> AGAIENARKEIKRISLEDHAESEYGAIYSVSGPVVIAENMIGCAMYELVKVGHDNLVGEVIRIDGDKATIQVYEETAGLTVGDPVLRTGKPLSVELGPGLMETIYDGIQRPLKAIKEESQSIYIPRGIDTPALDRTIKWQFTPGKFQVGDHISGGDIYGSVFENSLISSHKILLPPRSRGTITWIAPAGEYTLDEKILEVEFDGKKSDFTLYHTWPVRVPRPVTEKLSADYPLLTGQRVLDALFPCVQGGTTCIPGAFGCGKTVISQSLSKYSNSDAIIYVGCGERGNEMAEVLMEFPELYTEMSGTKEPIMKRTTLVANTSNMPVAAREASIYTGITLAEYFRDQGKNVSMIADSSSRWAEALREISGRLGEMPADQGFPAYLGAKLASFYERAGKAVALGSPDRTGSVSIVAAVSPAGGDFSDPVTTATLGITQVFWGLDKKLAQRKHFPSINTSVSYSKYTNVLNKFYDSNYP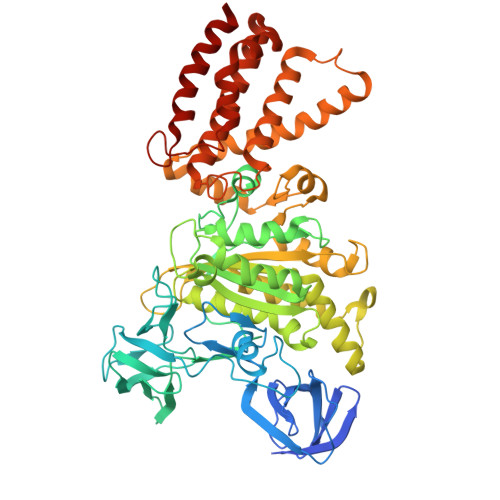EFPVLRDRMKEILSNAEELEQVVQLVGKSALSDSDKITLDVATLIKEDFLQQNGYSTYDAFCPIWKTFDMMRAFISYHDEAQKAVANGANWSKLADSTGDVKHAVSSSKFFEPSRGEKEVHGEFEKLLSTMQERFAESTD>MGSSHHHHHHSSGLVPAGSHSKVFIRSAINRVHQNSAANGGELPRIVFPEGTSTKVLKALATLVEEKICQPILLGYPERVKEKIKALDIPLLNDVSIVHPSSHPKYFSFVEKLYSLRQRKGINLGRAERLMADPNYFAAMMVNQGEADGMVSGSSINYADAVRPILQTIGVYKEGIPAGLNFVLLEDKFLVLADTTVNLNPTAEQCAQIALQAAKIVEYFGIEPRVAMLSYSNFSGAEGTPRKMKKAAEIARSLRPDLMIEGDMQADTAVNPEIMERLFPFSGLKGGANVLVFPNLESSNIAYKLIQQIGKAEVIGPFLTGVRRSANVLQRTTTVDGIVNSVVFTALEAQYIKEVLKSRGKK[6x]

Bacterial hybrid malic enzymes (MaeB grouping, multidomain) catalyse the transformation of malate to pyruvate, and are a major contributor to cellular reducing power and carbon flux. Distinct from other malic enzyme subtypes, the hybrid enzymes are regulated by acetyl-CoA, a molecular indicator of the metabolic state of the cell. The larger ME isoforms (hybrid enzymes) are predicted to be a fusion of two unrelated enzymes; a catalytic N-terminal ME subunit and a C-terminal phosphotransacetylase (PTA) domain. The PTA domain is homologous to PTA enzymes (that interconvert acetyl-CoA and phosphate to CoA and acetyl phosphate), yet they appear to lack critical catalytic residues and thus acts as a sensor instead.

The role of hexamerization was further validated by an E544R obligate dimer variant, which was insensitive to inhibition by acetyl-CoA.>[2x]MKTIGLVISTLNNPFFVTLKNGAEEKAKELGYKIIVEDSQNDSSKELSNVEDLIQQKVDVLLINPVDSDAVVTAIKEANSKNIPVITIDRSANGGDVVCHIASDNVKGGEMAAEFIAKALKGKGNVVELEGIPGASAARDRGKGFDEAIAKYPDIK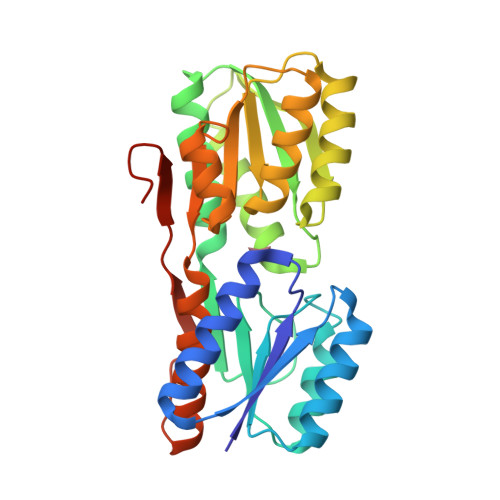IVAKQAADFDRSKGLSVMENILQAQPKIDAVFAQNDEMALGAIKAIEAANRQGIIVVGFDGTEDALKAIKEGKMAATIAQQPALMGSLGVEMADKYLKGEKIPNFIPAELKLITKENVQGSHHHHHH> MSFVITNPEALTVAATEVRRIRDRAIQSDAQVAPMTTAVRPPAADLVSEKAATFLVEYARKYRQTIAAAAVVLEEFAHALTTGADKYATAEADNIKTFSSGETHHHHHH;> MHFEAYPPEVNSANIYAGPGPDSMLAAARAWRSLDVEMT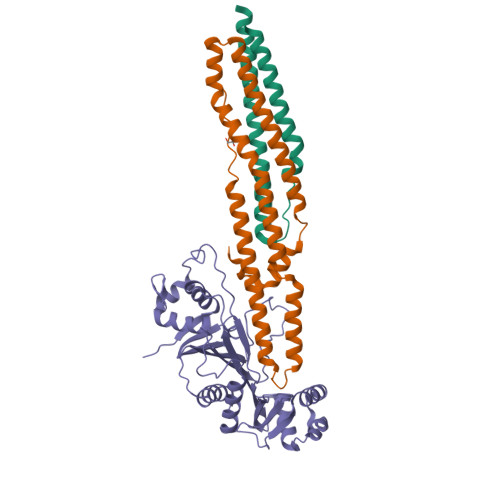AVQRSFNRTLLSLMDAWAGPVVMQLMEAAKPFVRWLTDLCVQLSEVERQIHEIVRAYEWAHHDMVPLAQIYNNRAERQILIDNNALGQFTAQIADLDQEYDDFWDEDGEVMRDYRLRVSDALSKLTPWKAPPPIA;> MDQQSTRTDITVNVDGFWMLQALLDIRHVAPELRCRPYVSTDSNDWLNEHPGMAVMREQGIVVNDAVNEQVAARMKVLAAPDLEVVALLSRGKLLYGVIDDENQPPGSRDIPDNEFRVVLARRGQHWVSAVRVGNDITVDDVTVSDSASIAALVMDGLESIHHADPAAINAVNVPMEEMLEATKSWQESGFNVFSGGDLRRMGISAATVAALGQALSDPAAEVAVYARQYRDDAKGPSASVLSLKDGSGGRIALYQQARTAGSGEAWLAICPATPQLVQVGVKTVLDTLPYGEWKTHSRVSSGGGSGGGSGGGS> 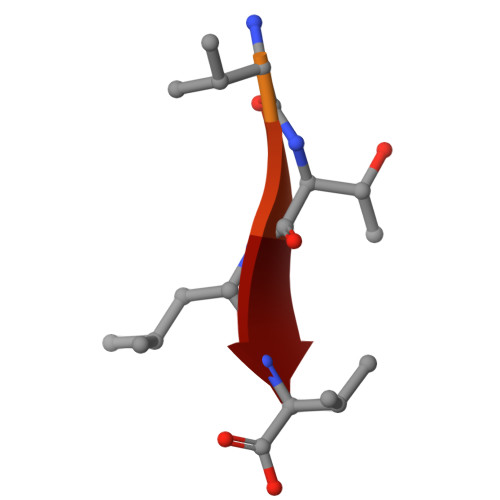YKVRNVTLV>[2x]MASSMRSLFSDHGKYVESFRRFLNHSTEHQCMQEFMDKKLPGIIGRIGDTKSEIKILSIGGGAGEIDLQILSKVQAQYPGVCINNEVVEPSAEQIAKYKELVAKISNLENVKFAWHKETSSEYQSRMLEKKELQKWDFIHMIQMLYYVKDIPATLKFFHSLLGTNAKMLIIV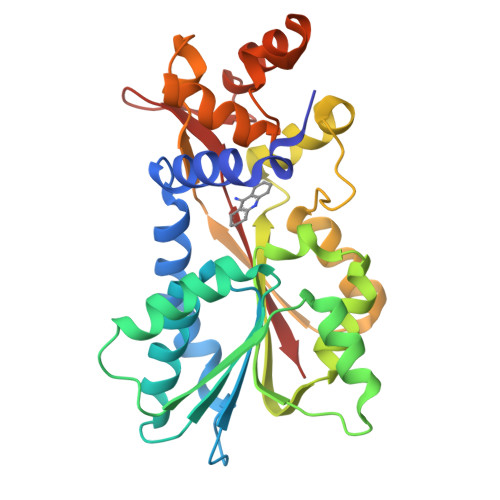VSGSSGWDKLWKKYGSRFPQDDLCQYITSDDLTQMLDNLGLKYECYDLLSTMDISDCFIDGNENGDLLWDFLTETCNFNATAPPDLRAELGKDLQEPEFSAKKEGKVLFNNTLSFIVIEA> XS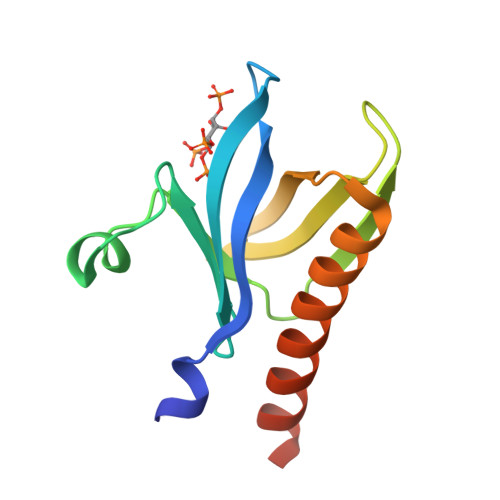MSDVAIVKEGWLHKRGEYIKTWRPRYFLLKNDGTFIGYKERPQDVDQREAPLNNFSVAQCQLMKTERPRPNTFIIRCLQWTTVIERTFHVETPEEREEWTTAIQTVADGLKKQEEEEMDFRSG>[4x]QIVTDNSIGNHDGYDYEFWKDSGGSGTMILNHGGTFSAQ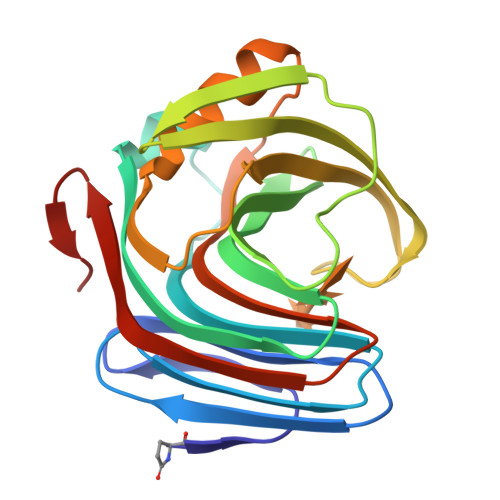WNNVNNILFRKGKKFNETQTHQQVGNMSINYGANFQPNGNAYLCVYGWTVDPLVAYYIVDSWGNWRPPGATPKGTITVDGGTYDIYETLRVNQPSIKGIATFKQYWSVRRSKRTSGTISVSNHFRAWENLGMNMGKMYEVALTVEGYQSSGSANVYSNTLRINGNPLSTI N-[(S)-({[(benzyloxy)carbonyl]amino}methyl)(hydroxy)phosphoryl]-N-methyl-L-leucinamide 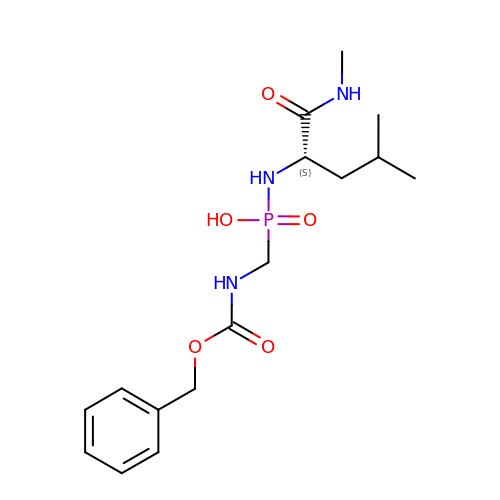| C16 H26 N3 O5 P | VZBGTFZRCJNJEQ-AWEZNQCLSA-N> NTVAAYNLTWKSTNFKTILEWEPKPVNQVYTVQISTKSGDWKSKCFYTTDTECDLTDEIVKDVKQTYLARV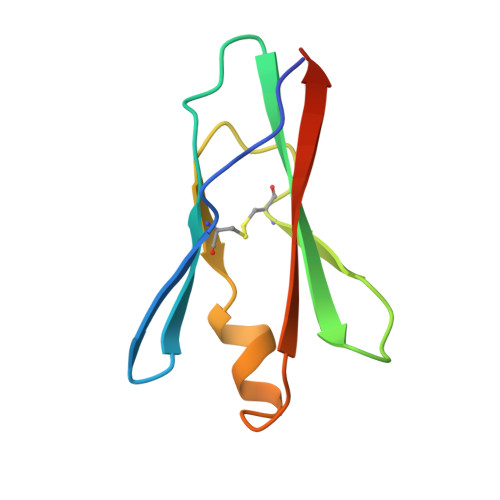FSYPAGNVE>[6x]MSITLRTYIFLDAL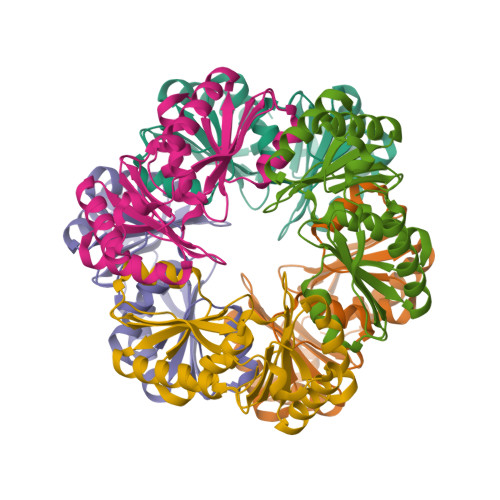QPQLATFIGKTARGFLPVPGQASLWVEIAPGIAINRVTDAALKATKVQPAVQVVERAYGLLEVHHFDQGEVLAAGSTILDKLEVREEGRLKPQVMTHQIIRAVEAYQTQIINRNSQGMMILPGESLFILETQPAGYAVLAANEAEKAANVHLVNVTPYGAFGRLYLAGSEAEIDAAAEAAEAAIRSVSGVAQESFRDR> MSEYSQTVPELVSWARKNDFSISLPVERLAFLMAIAVLNSERLDGEMSEGELIDAFREVCKGFEQTAESVAVRANNAINDMVRQKLLNRFTSELADGNAIYRLTPLGISISDYYIRQREFSTLRLSMQLSIVANELHRAAEAAEEGGDEFHWHRNVFAPLKYSVAEIFDSIDMSQRLMDEQQNFVKEDIAALLNQDWQAAIANCEQLLSETSGTLRELQDTLEAAGDKLQANLLRIQDANMGSGGSELVDKLVFDLQSKLDRIISWGQQAIDLWIGYDRHVHKFIRTAIDMDKNRIFSQRLRQSVQHYFDNPWTLTVANAERLLDMRDEELALRNEEVTGELPLELEYEEFSEINDQLAAMIEKALLVYQQEQRPLDLGAVLRDYLAQHPLPRHFDVARILVD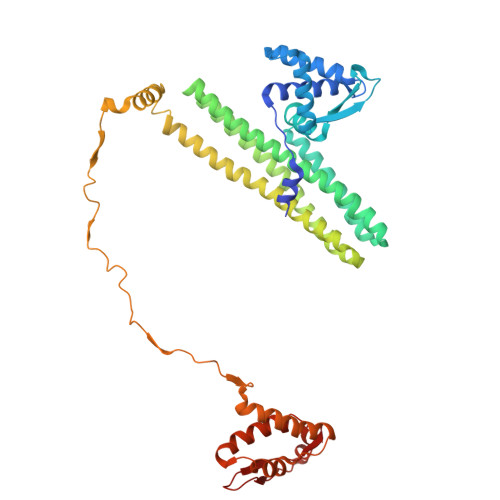QAVRLGVAEADFSGLPAEWLAINDYGAKVQAHVIDTY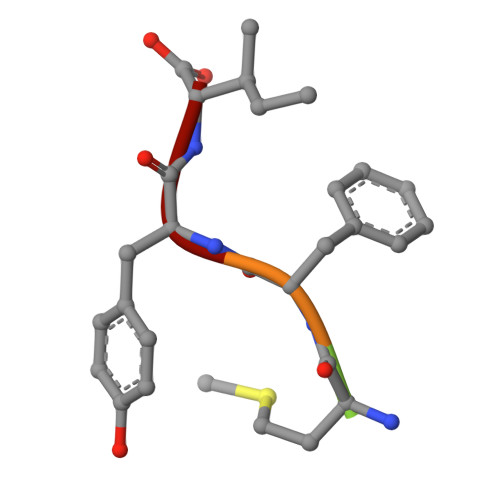> YMFYI>[3x]MQSEQWRSLSNVVWGKDLPAFTYAFSKTPLVLYDGGTTKQVGTYNFPVSKGMAGVYMSLEPGAIRELHWHANAAEWAYVMEGRTRITLTSPEGKVEIADVDKGGLWYFPRGWGHSIEGIGPDTAKFLLVF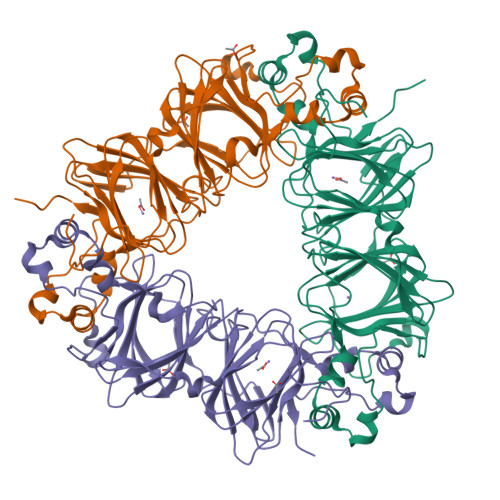NDGTFSEGATFSVTDWLSHTPIAWVEENLGWTAAQVAQLPKKQVYISSYGPASGPLASATPQGQTAKIEVPHTHNLLGQQPLVSLGGNELRLASAKEFPGSFNMTGALIHLEPGAMRQLHWHPNADEWQYVLDGEMDLTVFASEGKASVSRLQQGDVGYVPKGYGHAIRNSSQKPLDIVVVFNDGDYQSIDLSTWLASNPSSVLGNTFQISPELTKKLPVQDTIFSLPTQP>[2x]MRVTGVLREIVAHLREEIAERKRRVPLDELRARAASAPPPLDFLAALRGPRIRLIACIVGADPSVGAIRPEFDPAAIARSYEKAGAAAIGVFTIEDYFRGSDEYLQQVRAAVSLPVLRIDFIIDPYQVYEARALGADAILLLAAILSPAQLRELMAL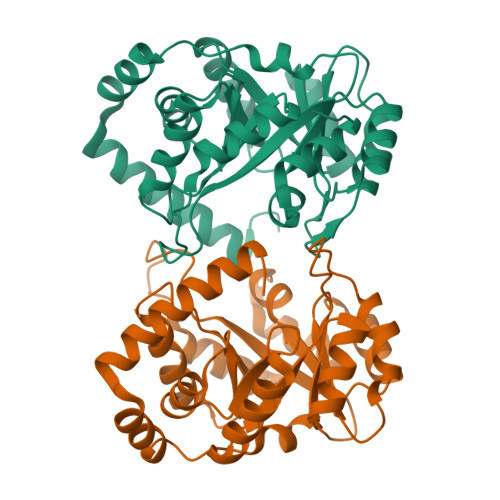AHELGMAAMVEVTDEEDVERALAAKAPLIVIINLNWDTLEISLETTRRLRQRIPPGITVVTWGGIHTREQVEEMEKLGVHAFMVMVALMRAPDPAAKVRELLGIGR> SAMGNSTGIKLVRKEGGLDDSVFIAVKEIGRDLYRGLPTEERIQKLEFMLDKLQNEIDQELEHNNSLVREEKETTDTRKKSLLSAALAKSGERLQALTLLMIHYRAGIEDIETLESLSLDQHSK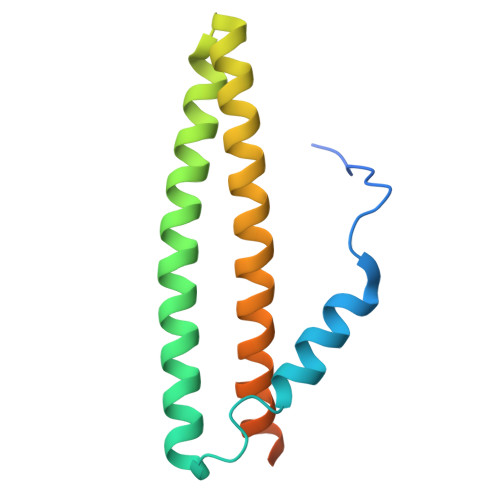KISKYTDDT>[4x]MSQHNEKNPHQHQSPLHDSSEAKPGMDSLAPEDGSHRPAAEPTPPGAQPTAPGSLKAPDTRNEKLNSLEDVRKGSENYALTTNQGVRIADDQNSLRAGSRGPTLLEDFILREKITHFDHERIPERIVAARGSAAHGYFQPYKSLSDITKADFLSDPNKITPVFVRFSTVQGGAGSADTVRDIRGFATKFYTEEGIFDLVGNNTPIFFIQDAHKFPDFVHAVKPEPHWAIPQGQSAHDTFWDYVSLQPETLHNVMWAMSDRGIPRSYRTMEGFGIHTFRLINAEGKATFVRFHWKPLAGKASLVWDEAQKLTGRDPDFHRRELWEAIEAGDFPEYELGFQLIPEEDEFKFDFDLL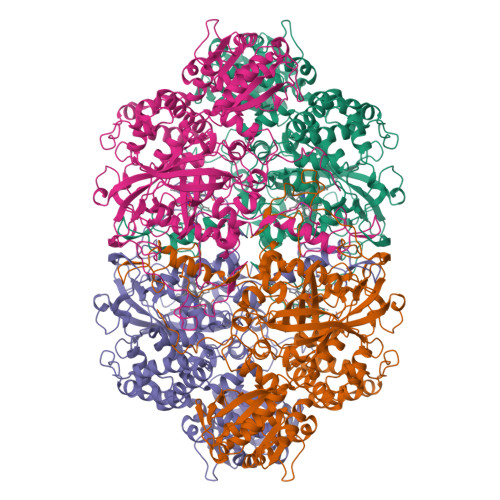DPTKLIPEELVPVQRVGKMVLNRNPDNFFAENEQAAFHPGHIVPGLDFTNDPLLQGRLFSYTDTQISRLGGPNFHEIPINRPTCPYHNFQRDGMHRMGIDTNPANYEPNSINDNWPRETPPGPKRGGFESYQERVEGNKVRERSPSFGEYYSHPRLFWLSQTPFEQRHIVDGFSFELSKVVRPYIRERVVDQLAHIDLTLAQAVAKNLGIELTDDQLNITPPPDVNGLKKDPSLSLYAIPDGDVKGRVVAILLNDEVRSADLLAILKALKAKGVHAKLLYSRMGEVTADDGTVLPIAATFAGAPSLTVDAVIVPCGNIADIADNGDANYYLMEAYKHLKPIALAGDARKFKATIKIADQGEEGIVEADSADGSFMDELLTLMAAHRVWSRIPKIDKIPA>NLYQFKNMIKCTVPSRSWWDFADYGCYCGRGGSGTPVDDLDRCCQVHDNCYNEAEKISGCWPYFKTYSYECSQGTLTCKG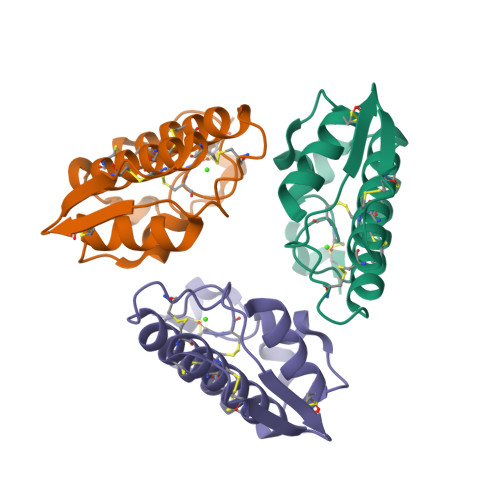DNNACAASVCDCDRLAAICFAGAPYNDNNYNIDLKARCQ[3x]> MHNHNHNHNHNHNGGENLYFQGASLTEIEHLVQSVCKSYRETCQLRLEDLLRQRSNIFSREEVTGYQRKSMWEMWERCAHHLTEAIQYVVEFAKRLSGFMELCQNDQIVLLKAGAMEVVLVRMCRAYNADNRTVFFEGKYGGMELFRALGCSELISSIFDFSHSLSALHFSEDEIALYTALVLINAHRPGLQE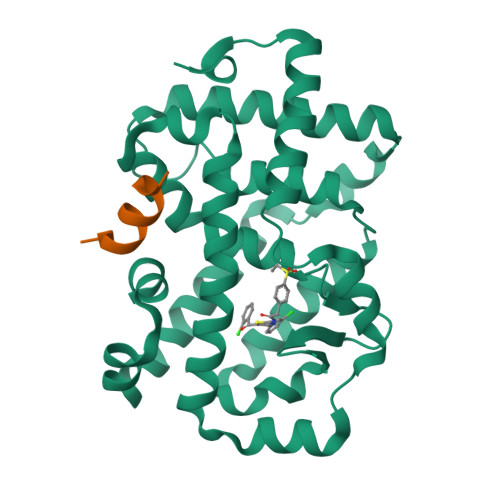KRKVEQLQYNLELAFHHHLCKTHRQSILAKLPPKGKLRSLCSQHVERLQIFQHLHPIVVQAAFPPLYKELFSGGSGGSGGKEKHKILHRLLQDSS;> KEKHKILHRLLQDSS>MADDVDNDDKLEKPVDLIWGCELNEQNKTFEFKVEDDEEKCEHQLALRTVCLGDKAKDEFHIVEIVDQEEGAEKSVPIATLKPSILPMATMVGIELDPPVTFRLKAGSGPLYISGQHVAM[9x];> MADDVDNDDKLEKPVDLIWGCELNEQNKTFEFKVEDDEEKCEHQLALRTVCLGDKAKDEFHIVEIVDQEEGAEKVVPIATLKPSILPMATMVGIELDPPVTFRLKAGS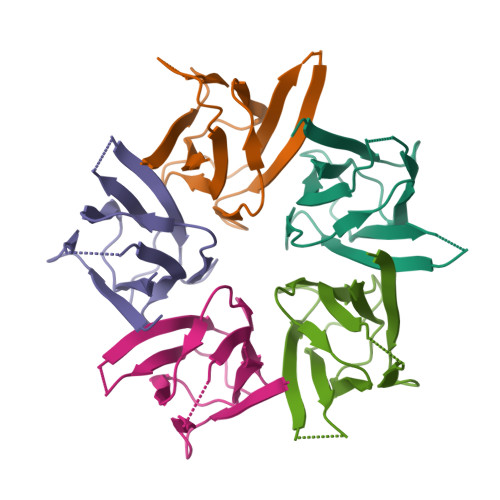GPLYISGQHVAM>MNLIPTVIETTNRGERAYDIYSRLLKDRIIMLGSQIDDNVANSIVSQLLFLQAQDSEKDIYLYINSPGGSVTAGFAIYDTIQHIKPDVQTICIGMAASMGSFLLAAGAKGKRFALPNAEVMIHQPLGGAQGQATEIEIAANHILKTREKLNRILSERTGQSIEKIQKDTD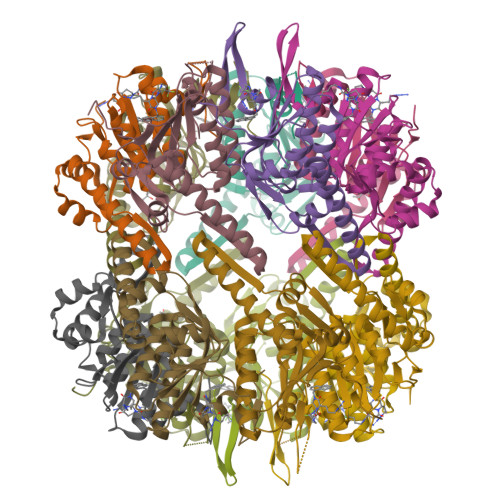RDNFLTAEEAKEYGLIDEVMVPETKHHHHHH[14x]>SMSNFVNLDIFSNYQKYIDNEQEVRENIRIVVREIEHLSKEAQIKLQIIHSDLSQISAACGLARKQVELCAQKYQKLAELVPAGQYYRYSDHWTFITQRLIFIIALVIYLEAGFLVTRETVAEMLGLKISQSEGFHLDVEDYLLGILQLASELSRFATNSVTMGDYERPLNISHFIGDLNTGFRLLNLKNDGLRKRFDALKYDVKKIEEVVYDVSIRG[2x];> IVQQFRIYSNELIMKHDRHERIVKLSRDITIESKRIIFLL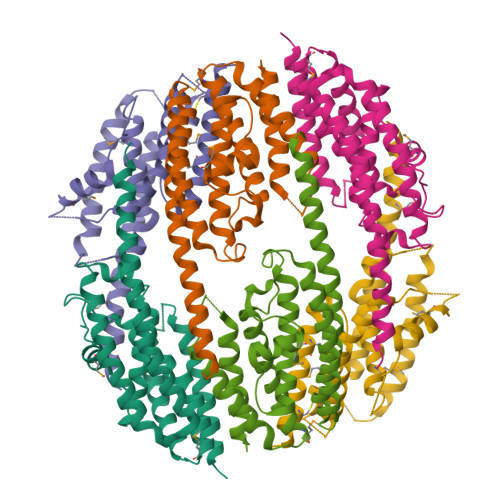HSIDSRKQNKEKVLEEARQRLNKLIAVNFRAVALELRDQDVYQFRSSYSPGLQEFIEAYTYMEYLCHEDAEGENETKSVSDWQAIQAVMQYVEESSQPKEEPTEGEDVQAIAQVESPKKFQFFVDPTEYILGLSDLTGELMRRCINSLGSGDTDTCLDTCKALQHFYSGYISLNCQRARELWRKITTMKQSVLKAENVCYNVKVRGGEAAKWGATFDQKPADEVDEGFY> ANVSFSLSGADSKSYSKFITALRKALPSKEKVSNIPLLLPSASGASRYILMQLSNYDAKAITMAIDVTNV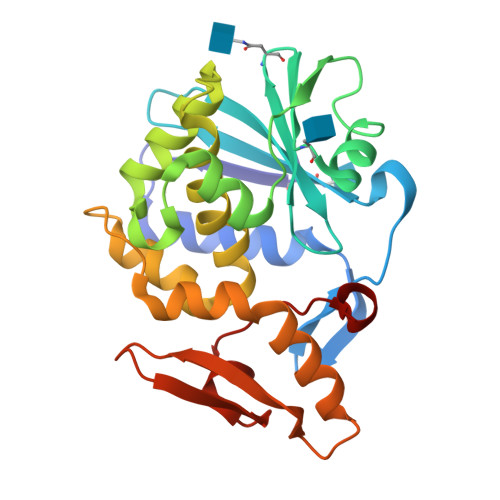YIMGYLVNSTSYFFNESDAKLASQYVFKGSTIVTLPYSGNYERLQNAAGKVREKIPLGFRAFDSAITSLFHYDSTAAAGAFLVIIQTTAEASRFKYIEGQIIKRIPKNEVPSPAALSLENEWSALSKQIQLAQTNNGAFRTPVVIIDNKGQRVEIKDVNSKVVTNNIKLLLNKQNIA>SEISRQEFQRRRQALVEQMQPGSAALIFAAPEVTRSADSEYPYRQNSDFWYFTGFNEPEAVLVLIKSDDTHNHSVLFNRVRDLTAEIWFGRRLGQDAAPEKLGVDRALAFSEINQQLYQLLNGLDVVYHAQGEYAYADVIVNSALEKLRKGSRQNLTAPATMIDWRPVVHEMRLFKSPEEIAVLRRAGEITAMAHTRAMEKCRPGMFEYHLEGEIHHEFNRHGARYPSYNTIVGSGENGCILHYTENECEMRDGDLVLIDAGCEYKGYAGDITRTFPVNGKFTQAQREIYDIVLESLETSLRLYRPGTSILEVTGEVVRIMVSGLVKLGILKGDVDELIAQNAHRPFFMHGLSHWLGLDVHDVGVYGQDRSRILEPGMVLTVEPGLYIAPDAEVPEQYRGIGIRIEDD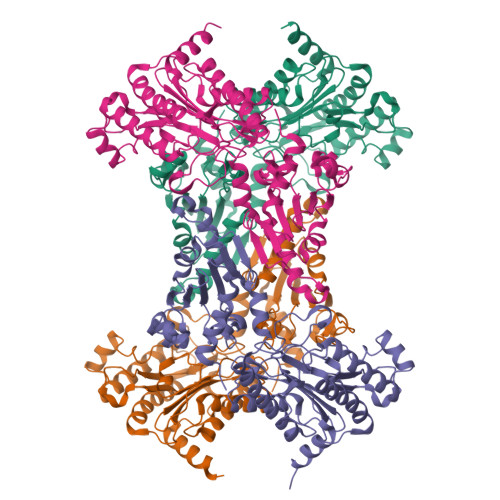IVITETGNENLTASVVKKPEEIEALMVAARKQ[6x]> CPQEDSDIAFLIDGSGSIIPHDFRRMK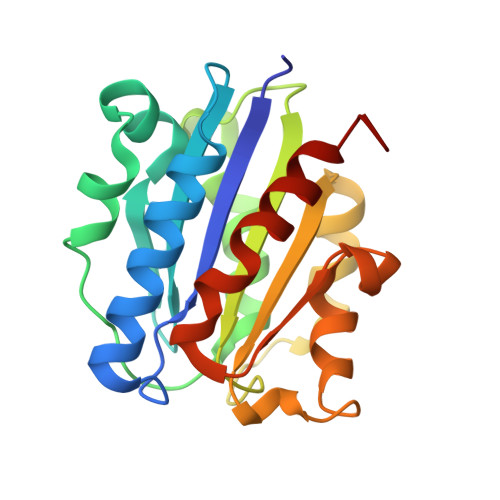EFVSTVMEQLKKSKTLFSLMQYSEEFRIHFTFKEFQNNPNPRSLVKPITQLLGRTHTATGIRKVVRELFNITNGARKNAFKILVVITDGEKFGDPLGYEDVIPEADREGVIRYVIGVGDAFRSEKSRQELNTIASKPPRDHVFQVNNFEALKTIQNQLREKIFAIGSPGI> GSTIQPGTGYNN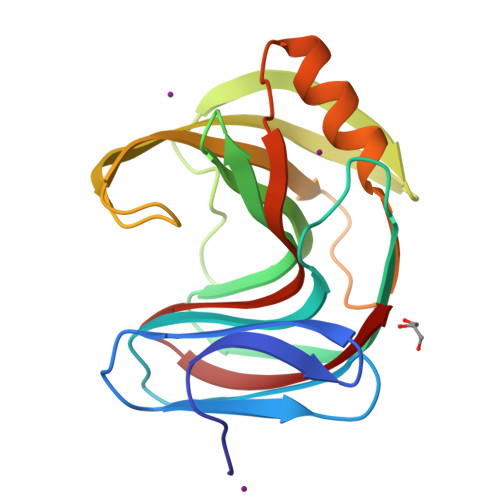GYFYSYWNDGHGGVTYTNGPGGQFSVNWSNSGEFVGGKGWQPGTKNKVINFSGSYNPNGNSYLSVYGWSRNPLIEYYIVENFGTYNPSTGATKLGEVTSDGSVYDIYRTQRVNQPSIIGTATFYQYWSVRRNHRSSGSVNTANHFNAWAQQGLTLGTMDYQIVAVQGYFSSGSASITVS>MSIDWEQTFRKWSKPSSETESTKAENAERMIKAAINSSQILSTKDISVFPQGSYRNNTNVREDSDVDICVCLNTLVLSDYSLVPGMNDKLAELRTASYTYKQFKSDLETALKNKFGTLGVSRGDKAFDVHANSYRVDADVVPAIQGRLYYDKNHNAFIRGTCIKPDSGGTIYNWPEQNYSNGVNKNKSTGNRFKLIVRAIKRLRNHLAEKGYNTAKPIPSYLMECLVYIVPDQYFTGDSYKTNVENCINYLYNQIDSSDWTEINEIKYLFGSHQMW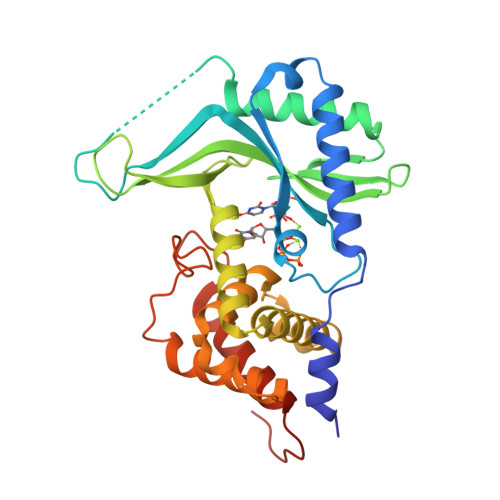NKTQVKEFLLTAWSYIQKNLEHHHHHH[2x]> HQLYIDETVNSNIPTNLRVLRSILENLRSKIQKLESDVSAQMEYCRTPCTVSCNIPVVSGKECEEIIRKGGETSEMYLIQPDSSVKPYRVYCDMNTENGGWTVIQNRQDGSVDFGRKWDPYKQGFGNVATNTDGKNYCGLPGEYWLGNDKISQLTRMGPTELLIEMEDWKGDKVKAHYGGFTVQNEANKYQISVNKYRGTAGNALMDGA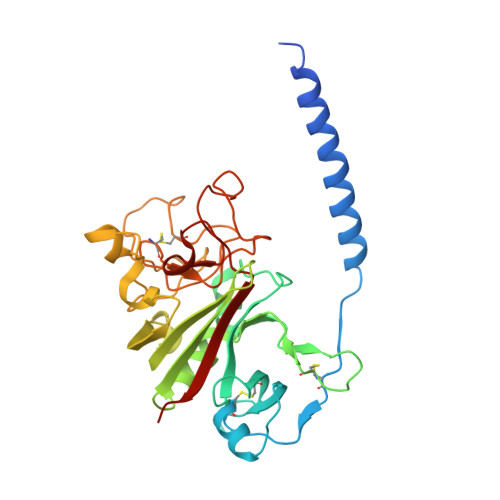SQLMGENRTMTIHNGMFFSTYDRDNDGWLTSDPRKQCSKEAGGGWWYNRCHAANPNGRYYWGGQYTWDMAKHGTDDGVVWMNWKGSWYSMRKMSMKIRPFFPQQ> MVPISPIETVPVKLKPGMDGPKVKQWPLTEEKIKALVEICTEMEKEGKISKIGPENPYNTPVFAIKKKDSTKWRKLVDFRELNKRTQDFWEVQLGIPHPAGLKKKKSVTVLDVGDAYFSVPLDEDFRKYTAFTIPSINNETPGIRYQYNVLPQGWKGSPAIFQSSMTKILEPFKKQNPDIVIYQYMDDLYVGSDLEIGQHRTKIEELRQHLLRWGLTTPDKKHQKEPPFLWMG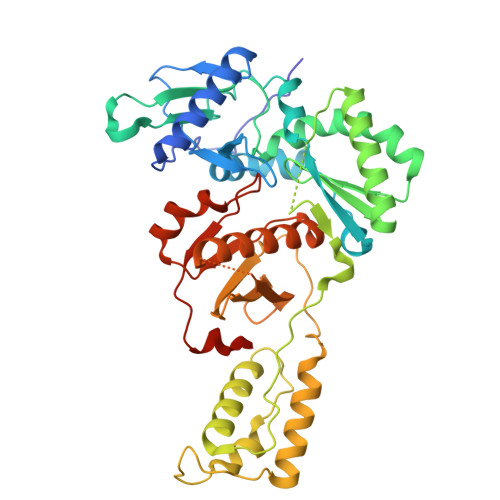YELHPDKWTVQPIVLPEKDSWTVNDIQKLVGKLNWASQIYPGIKVRQLSKLLRGTKALTEVIPLTEEAELELAENREILKEPVHGVYYDPSKDLIAEIQKQGQGQWTYQIYQEPFKNLKTGKYARMRGAHTNDVKQLTEAVQKITTESIVIWGKTPKFKLPIQKETWETWWTEYWQATWIPEWEFVNTPPLVKLWYQLEKEPIVGAETF>LTAKHRPSVVWLHNAECGGCTEAAIRTIKPYIDALILDTISLDYQETIMAAAGEAAEAALHQALEGKDGYYLVVEGGLPTIDGGQWGMVAGHPMIETTKKAAAKAKGIICIGTCSAYGGVQKAKPNPSQAKGVSEALGVKTINIPGCPPNPINFVGAVVHVLTKGIPDLDENGRPKLFYGELVHDNCPRLPHFEASEFAPSFDSEEAKKGFCLYELGCKGPVTYNNCPKVLFNQVNWPVQAGHPCLGCSEPDFWDTMTPFYEQG[3x];>ASWSHPQFEKGASGAAESKPTPQSTFTGPIVVDPITRIEGHLRIMVEVENGKVKDAWSSSQLFRGLEIILKGRDPRDAQHFTQRACGVCTYVHALASSRCVDDAVKVSIPANARMMRNLVMASQYLHDHLVHFYHLHALDWVDVTAALKADPNKAAKLAASIAPARPGNSAKALKAVQDKLKAFVESGQLGIFTNAYFLGGHKAYYLPPEVDLIATAHYLEALHMQVKAASAMAILGGKNPHTQFTVVGGCSNYQGLTKDPLANYLALSKEVCQFVNECYIPDLLAVAGFYKDWGGIGGTSNYLAFGEFATDDSSPEKHLATSQFPSGVITGRDLGKVDNVDLGAIYEDVKYSWYAPGGDGKHPYDGVTDPKYTKLDDKDHYSWMKAPRYKGKAMEVGPLARTFIAYAKGQPDFKKVVDMVLGKLSVPATALHSTLGRTAARGIETAIVCANMEKWIKEMADSGAKDNTLCAKWEMPEESKGVGLADAPRGALSHWIRIKGKKIDNFQLVVPSTWNLGPRGAQGDKSPVEEALIGTPIADPKRPVEILRTVHAFDPCIACGVH[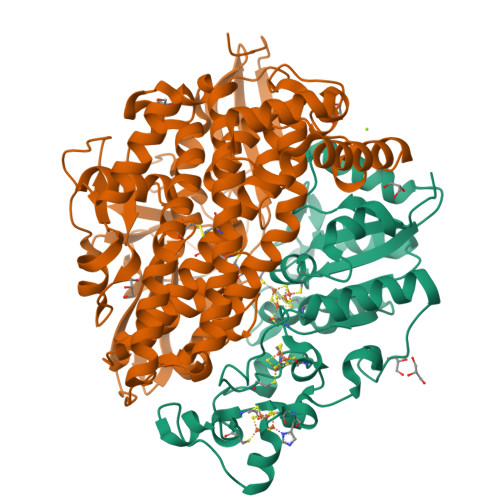3x]> MSTKAEQFASKIRYLQEYHNRVLHNIYPVPSGTDIANTLKYFSQTLLSVLRDAPSERGPQSRDAQLSDYPSLDYQGLYVTLVTLLDLVPLLQHGQHDLGQSIFYTTTCLLPFLNDDVLSTLPYTMISTLATFPPFLHKDIIEYLSTSFLPMAILGSSGREGVPAHVNLSASSMLMIAMQYTSNPVYHCQLLECLMKYKQEVWKDLLYVIAYGPSQVKPPAVQMLFHYWPNLKPPGAISEYRGLQYTAWNPIHCQHIECHNAINKPAVKMCIDPSLSVALGDKPPPLYLCEECSERISGDHSEWLIDVLLPQAEISAICQKKNCSSHVRRAVVTCFSAGCCGRHGNRPVRYCKRCHSNHHSNEVGATAETHLYQTSPPPINTRECGAEELVCAVEAVISLLKEAEFHAEQREHELNRRRQLGLSSSHHSLDNTDFDNKDDDKHDQRLLSQFGIWFLVSLCTPSENTPTESLARLVAMVFQWFHSTAYMMDDEVGSLVEKLKPQFVTKWLKTVCDVRFDVMVMCLLPKPMEFARVGGYWDKSCSTVTQLKEGLNRILCLIPYNVISQSVWECIMPEWLEAIRTEVPDNQLKEFREVLSKMFDIELCPLPFSMEEMFGFISCRFTGYPSTVQEQALLWLHVLSELDITVPLQLLISMFSDGVNSVKELANQRKSRANELAGNLASRRVSVASDPGRRGQHNTLSPFHSPFQSPFRSPMRSPFRSPFKNFGHPGGRTIDFDCEDDDMNLNCFILMFDLLLKQMELQDDGITMGLEHSLSKDIISIINNVFQAPWGGSHSCQKDKKATECNLCQSSILCYQLACELLERLAPKEESRLVEPTDSLEDSLLSSRPEFILGPEGEEEENPAAKHGENPGNRTVPSEHAAIKNDTERKFCYQQLPVTLRLIYTIFQEMAKFEEPDILFNMLNCLKILCLHGECLYTARKDHPQFLAYIQDHMLIASLWRVVKSEFSQLSSLAVPLLLHALSLPHGADIFWTIINGNFNSKDWKMRFEAVEKVAVICRFLDIHSVTKNHLLKYSLAHAFCCFLTAVEDVNPAVATRAGLLLDTIKRPALQGLCLCLDFQFDTVVKDRPTILSKLLLLHFLKQDIPALSWEFFVNRFETLSLEAQLHLDCNKEFPFPTTITAVRTNVANLSDAALWKIKRARFARNRQKSVRSLRDSVKGPAESKRALSLPETLTSKIPVRLTRHEQSAPALGGTPEQTPGQQSPENDNTIKDLLPEDAGIDHQTVHQLITVLMKFMARDESSAESDISSAKAFNTVKRHLYVLLGYDQQEGCFMIAPQKMRLSTCFNAFIAGIAQVMDYNINLGKHLLPLVVQVLKYCSCPQLRHYFQQPPRCSLWSLKPHIRQMWLKALLVILYKYPYRDCDVSKTLLHLIHITVNTLNAQYHSCKPHATAGPLYTDNSNISRYSEKEKEEDSVFDESDIHDTPTGPCNKESQTFFARLKRIGGSRMVKGQPVGMNVQRSEIELAEYRETGALQDSVLHCVREESIQKKKLRSLKQKSLDIGNADSLLFTLDEHRRKSCIDRCDIDKPPAQAAYISQRQNDHHGRSRQNSATRPDNTEIPKNPGTEGFQEIRRPVIPEVRLNCMETFEVRVDSPGKPAPREDLDLIDLSSDSTSGPEKHSILSTSDSDSLVFEPLPPLRIVESDEEEEMMNQGNGGALGNNAASSPSIPSQPSVLSLSTTPLVQVSVEDCSKDFSSKDSGNHQSASNEDSTIAALDDLTDSEELSKSEELREFASGSPLTLKQKRDLLQKSSAVPEMSVDYNPEPSPAEEKPGQTPTSGVKTVLLKVPEDGENLIESEKPNTSAESDTEQNPERKVEEDGAEESEFKIQIVPRQRKQRKIAVSAIQREYLDISFNILDKLGEQKDPDPSAKGLSTLEMPRESSSAPTLEAGAPETSSHSSISTQYRQMKRGSLGVLTMSQLMKRQLEHQSSAPHNISSWDTEQIQPGKRQCNVPMCLNPDLEGQPLRTRGATKSSLLSAPSIASMFVPAPEEFTEEQPTVMADKCHDCGAILEEYDEETLGLAIVVLSTFIHLSPDLAAPLLLDIMQSVGRLASSTTFSNQAESMMVPGNAAGVAKQFLRCIFHQLAPNGIFPQLFQSAIKDGTFLRTLATSLMDFNELSSIAALSQLLEGLNNKKNLPAGGAMIRCLENIATFMEALPMDSPSSLWTTISNQFQTFFAKLPCVLPLKCSLDSSLRIMICLLKIPSTNATRSLLEPFSKLLSFVIQNAVFTLAYLVELCGLCYRAFTKERDKFYLSRSVVLELLQALKLKSPLPDTNLLLLVQFICADAGTKLAESTILSKQMIASVPGCGTAAMECIRQYVSEVLEFMADMHTLTKLKSHMKTCSQPLHEDTFGGHLKVGLAQIAAMEISRGNHRDNKAVIRYLPWLYHPPSAMQQGPKEFIECVSHIRLLSWLLLGSLTHNAVCPNASSPCLPIPLDAGSHIADHLIVILIGFPEQSKTCVLHMCSLFHAFIFAQLWTVYCEQSAVATNVQNQNEFSFTAILTALEFWSRVTPSILQLMAHNKVMVEMVCLHVISLMEALQECNSTIFVKLIPMWLPMIQSNTKHLSAGLQLRLQAIQNNVNHHSLRTLPGSGQSSAGLAALRKWLQCTQFKMAQVEIQSSEAASQFYPL;> MVKRKSSEGQEQDGGRGIPLPIQTFLWRQTSAFLRPKLGKQYEASCVSFERVLVENKLHGLSPALSEAIQSISRWELVQAALPHVLHCTATLLSNRNKLGHQDKLGVAETKLLHTLHWMLLEAPQDCNNDQFGGTDRGSSWGGSSSAFIHQIENQGSPGQPCRSSSHDEEENNRRKTFQNSMATVELFVFLFAPLVHRIKESDLTFRLASGLVIWQPMWEHRQPEVSGFTALVKPIRNIITAKRSSPINSQSQTCESPNQDTRQQGEGLQVVSEALQSDSISPKATISGCHQGNSFDGSLSSQTSQERGPSHSRASLVIPPCQRSRYATYFDVAVLRCLLQPHWSEEGTQWSLMYYLQRLRHMLEEKPEKTPDPDIPLLPRPRSSSMVAAAPSLVNTHKTQDLTMKCNEEEKSLSPEAFSKVSLTNLRRSAVPDLSSDLGMNIFKKFKSRKEDRERKGSIPFHHTGKRRPRRMGVPFLLHEDHLDVSPTRSTFSFGSFSGLGEDRRGIEKGGWQTTILGKLTRRGSSDAATEMESLSARHSHSHHTLVSDLPDHSNSHGENTVKEVRSQISTITVATFNTTLASFNVGYADFFSEHMRKLCSQVPIPEMPHEPLACANLPRSLTDSCINYSYLEDTEHIDGTNNFVHKNGMLDLSVVLKAVYLVLNHDISSRICDVALNIVECLLQLGVVPCVEKNRKKSENKENESVEKRPSEGAFQFKGVSSSSTSGFGAPSASGAGDGGGEEGGGGDGGGGGGGGDGGGGGGGGGGPYEKNEKNQEKDDNIPVSNHRLALTMLIKIVKSLGCAYGCGEGHRGLSGDRLRHQVFRENAQNCLTKLYKLDKIQFRQTMRDYVNKDSLNNVVDFLHALLGFCMEPVTDNKAGFGNNFTTVDNKSTAQNVEGIIVGAMFKSLITRCASTTHELHSPENLGLYCDIRQLVQFIKEAHGNVFRRVALSALLDSAEKLAPGKKVEENGQESKPVGSKRSEAGSIADKGQVSSAPEECRSFMSGRPSQTPEHDEPMQGGNLGRKDFWRKMFKSQSAASDTSSQSEQDTSECTTAHSGNTSDRRARSRSRRISLRKKLKLPIGNWLKRSSLSGLADGVEDLLDISSVDRLSFIRQSSKVKFTSAVKLSEGGPGSGMENGREEEENFFKRLGCHSFDDHLSPNQDGGKSKNVVNLGAIRQGMKRFQFLLNCCEPGTIPDASILAAALDLEAPVVARAALFLECARFVHRCNRGNWPEWMKGHHVNITKKGLSRGRSPTVGNKRNQKLQWSAAKLFYQWGDAIGIRLNELCHGESESPANLLGLIYDEETKRRLRKEDEEEDFLDDSTVNPSKCGCPFALKMAACQLLLEITTFLRETFSCLPRPRTEPLVDLESCRLRLDPELDRHRYERKISFAGVLDENEDSKDSLHSSSHTIKSDAGAEEKKVPSRKIRIGGSRLLQIKGTRSFQVKKGGSLSSIRRVGSLKSSKLSRQDSESEAEELQLSQSRDTVTDLEGSPWSASEPSIEPEGLSNAGTEENYHRNMSWLHVMILLCNQQSFICTHVDYCHPHCYLHHSRSCARLVRAIKLLYGDSVDSLRESNHISNVALRGKKQKECSDKSCLRTPSLKKRVSDVNLEGKKDSGMLKYIRFQVMSLSPAPLSLLIKAAPILTEEMYGDIQPAAWELLLSMDEHMAGAAAAMFLLCAVKVPDAVSDMLMSEFHHAETVQRLNAVLKFHTLWRFRYQVWPRMEEGAQQIFKIPPPSINFTLPSPVLGMPSVPMFDPPWVPQCSGSVQDPINEDQSKSFSARAVSRSHQRAEHILKNLQQEEEKKRLGREASLITAIPITQEACYEPTCTPNSEPEEEEEVANLTSRRLSVSPSCTSSTSHRNYSFRRGSVWSVRSAVSAEDEEHATEHTPNHHVPQPPQAVFPACICAAVLPIVHLMEDGEVREDGVAVSAVAQQVLWNCLIEDPSTVLRHFLEKLTISNRQDELMYMLRKLLLNIGDFPAQTSHILFNYLVGLIMYFVRTPCEWGMDAISATLTFLWEVVGYVEGLFFKDLKQTMKKEQCEVKLLVTASMPGTKTLVVHGQNECDIPTQLPVHEDTQFEALLKECLEFFNIPESQSTHYFLMDKRWNLIHYNK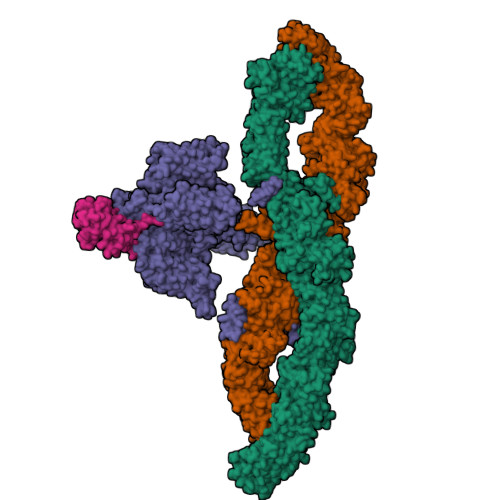TYVRDIYPFRRSVSPQLNLVHMHPEKGQELIQKQVFTRKLEEVGRVLFLISLTQKIPTAHKQSHVSMLQEDLLRLPSFPRSAIDAEFSLFSDPQAGKELFGLDTLQKSLWIQLLEEMFLGMPSEFPWGDEIMLFLNVFNGALILHPEDSALLRQYAATVINTAVHFNHLFSLSGYQWILPTMLQVYSDYESNPQLRRAIEFACHQFYILHRKPFVLQLFASVAPLLEFPDAANTGSSKGVSAQCLFDLLQSLEGETTDILDILELVKAEKPLKSLDFCYGNEDLTFSISEAIKLCVTVVAYAPESFRSLQMLMVLEALVPCYLQKMKRQTSQVETVPAAREEIAATAALATSLQALLYSVEVLTRPMTAPQMSRSDQGHKGTTTANHTMSSGVNTRYPEQGAKLHFIRENLHLLEEGQGLPREELDERISREEFRRPRESLLNICTEFYKHCGPRLKILQNLAGEPRVTALELLDVKSHMRLAEIAHSLLKLAPYDTQTMESRGLRRYIMEMLPITDWSAEAVRPALILILKRLDRMFNKIHKMPTLRRQVEWEPASSLIEGVCLTLQRQPIISFLPHLRSLINVCVNLVMGVVGPSSVADGLPLLHLSPYLSPPLPFSTAVVRLVALQIQALKEDFPLSHVISPFTNQERREGMLLNLLIPFVLTVGSGSKDSPWLEQPEVQLLLQTVINVLLPPRIISTSRSKNFMLESSPAHCSTPGDAGKDLRKEGLAESTSQAAYLALKVILVCFERQLGSQWYWLSLQVKEMALRKVGGLALWDFLDFIVRTRIPIFVLLRPFIQCKLLAQPAENHEELSARQHISDQLERRFIPRPLCKSSLIAEFNSELKILKEAVHSGSAYQGKTSISTVGTSTSAYRLSLATMSRSNTGTGTVWEQDSEPSQQASQDTLSRTDEEDEENDSVSMPSVVSEQEACLLSTIGRRRFSSHVSSMSAPQAEVGMLPSQSEPNVLDDSQGLAAEGSLSRVASIQSEPGQQNVLLQQPLGRKRGLRQLRRPLLSRQKTQTEPRNRHGARLSTTRRSIQPKTKPSVDQKRSVTFIEAQPEPTAAPTDIFPATGQPQSCSPGRARKPEGTEKPVLTSSPAIIIADLHSLSPKQSEPLLAEEGEKKEDEEIQGATAHCPLSTQLSDPDDFTGLETSSLLQHGDTVLHISEENGTENPLLSSQFTFTPPELGDTDSALDESHV;> MLKRKQSSRVEAQPVTDFGPDESLSDNADILWINKPWVHSLLRICAIISVISVCMNTPMTFEHYPPLQYVTFTLDTLLMFLYTAEMIAKMHIRGIVKGDSSYVKDRWCVFDGFMVFCLWVSLVLQVFEIADIVDQMSPWGMLRIPRPLIMIRAFRIYFRFELPRTRITNILKRSGEQIWSVSIFLLFFLLLYGILGVQMFGTFTYHCVVNDTKPGNVTWNSLAIPDTHCSPELEEGYQCPPGFKCMDLEDLGLSRQELGYSGFNEIGTSIFTVYEASSQEGWVFLMYRAIDSFPRWRSYFYFITLIFFLAWLVKNVFIAVIIETFAEIRVQFQQMWGTRSSTTSTATTQMFHEDAAGGWQLVAVDVNKPQGRAPACLQKMMRSSVFHMFILSMVTVDVIVAASNYYKGENFRRQYDEFYLAEVAFTVLFDLEALLKIWCLGFTGYISSSLHKFELLLVIGTTLHVYPDLYHSQFTYFQVLRVVRLIKISPALEDFVYKIFGPGKKLGSLVVFTASLLIVMSAISLQMFCFVEELDRFTTFPRAFMSMFQILTQEGWVDVMDQTLNAVGHMWAPLVAIYFILYHLFATLILLSLFVAVILDNLELDEDLKKLKQLKQSEANADTKEKLPLRLRIFEKFPNRPQMVKISKLPSDFTVPKIRESFMKQFIDRQQQDTCCLFRILPSTSSSSCDNPKRPTVEDNKYIDQKLRKSVFSIRARNLLEKETAVTKILRACTRQRMLSGSFEGQPAKERSILSVQHHIRQERRSLRHGSNSQRISRGKSLETLTQDHSNTVRYRNAQREDSEIKMIQEKKEQAEMKRKVQEEELRENHPYFDKPLFIVGREHRFRNFCRVVVRARFNASKTDPVTGAVKNTKYHQLYDLLGLVTYLDWVMITVTICSCISMMFESPFRRVMHAPTLQIAEYVFVIFMSIELNLKIMADGLFFTPTAVIRDFGGVMDIFIYLVSLIFLCWMPQNVPAESGAQLLMVLRCLRPLRIFKLVPQMRKVVRELFSGFKEIFLVSILLLTLMLVFASFGVQLFAGKLAKCNDPNIIRREDCNGIFRINVSVSKNLNLKLRPGEKKPGFWVPRVWANPRNFNFDNVGNAMLALFEVLSLKGWVEVRDVIIHRVGPIHGIYIHVFVFLGCMIGLTLFVGVVIANFNENKGTALLTVDQRRWEDLKSRLKIAQPLHLPPRPDNDGFRAKMYDITQHPFFKRTIALLVLAQSVLLSVKWDVEDPVTVPLATMSVVFTFIFVLEVTMKIIAMSPAGFWQSRRNRYDLLVTSLGVVWVVLHFALLNAYTYMMGACVIVFRFFSICGKHVTLKMLLLTVVVSMYKSFFIIVGMFLLLLCYAFAGVVLFGTVKYGENINRHANFSSAGKAITVLFRIVTGEDWNKIMHDCMVQPPFCTPDEFTYWATDCGNYAGALMYFCSFYVIIAYIMLNLLVAIIVENFSLFYSTEEDQLLSYNDLRHFQIIWNMVDDKREGVIPTFRVKFLLRLLRGRLEVDLDKDKLLFKHMCYEMERLHNGGDVTFHDVLSMLSYRSVDIRKSLQLEELLAREQLEYTIEEEVAKQTIRMWLKKCLKRIRAKQQQSCSIIHSLRESQQQELSRFLNPPSIETTQPSEDTNANSQDHNTQPESSSQQQLLSPTLSDRGGSRQDAADTGKPQRKIGQWRLPSAPKPISHSVSSVNLRFGGRTTMKSVVCKMNPMPDTASCGSEVKKWWTRQLTVESDESGDDLLDI;> MTRGAWMCRQYDDGLKIWLAAPRENEKPFIDSERAQKWRLSLASLLFFTVLLSDHLWFCAEAKLTRTRDKEHHQQQQQQQQQQQQQQQQQQQQQQRQQQRQRQQQRQRQQEPSWPALLASMGESSPAAQAHRLLSASSSPTLPPSPGGGGGSKGNRGKNNRSRALFLGNSAKPVWRLETCYPQGASSGQCFTVESADAVCARNWSRGAAAGEEQSSRGSRPTPLWNLSDFYLSFCNSYTLWELFSGLSSPSTLNCSLDVVLTEGGEMTTCRQCIEAYQDYDHHAQEKYEEFESVLHKYLQSDEYSVKSCPEDCKIVYKAWLCSQYFEVTQFNCRKTIPCKQYCLEVQTRCPFILPDNDEVIYGGLSSFICTGLYETFLTNDEPECCDIRSEEQTAPRPKGTVDRRDSCPRTSLTVSSATRLCPGRLKLCVLVLILLHTVLTASAAQNSTGLGLGGLPTLEDNSTRED4-[(4-imidazo[1,2-a]pyridin-3-yl-1,3-thiazol-2-yl)amino]phenol 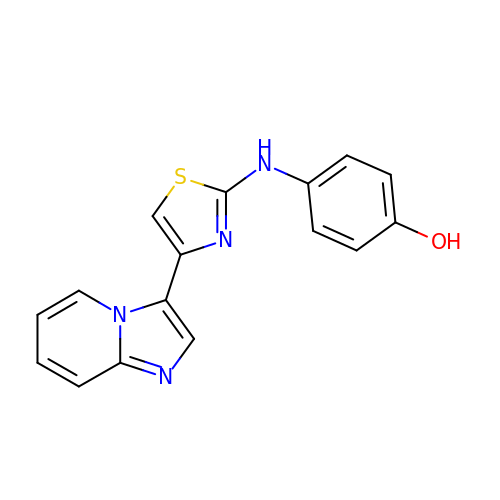| C16 H12 N4 O S | NAJHZKDVMWYLOU-UHFFFAOYSA-N> TQELGNANFENFIGATEGFSEIAYQFTSHILTLGYAVMLAGLLYFILTIKNVDKKFQMSNILSAVVMVSAFLLLYAQAQNWTSSFTFNEEVGRYFLDPSGDLFNNGYRYLNWLINVPMLLFQILFVVSLTTSKFSSVRNQFWFSGAMMIITGYIGQFYEVSNLTAFLVWGAISSAFFFHILWVMKKVINEGKEGISPAGQKILSNIWILFLISWTLYPGAYLMPYLTGVDGFLYSEDGVMARQLVYTIADVSSKVIYGVLLGNLAITLSKNKEL

Microbial rhodopsins (MRs) are transmembrane light-sensitive proteins, found in Archaea, Bacteria, Eukaryota, and also viruses. MRs are composed of seven transmembrane α-helices (A–G) with the cofactor retinal covalently bound to the lysine residue of helix G via the Schiff base (RSB). Despite this paradigm, the first light-driven Na+ pump KR2 was identified in Krokinobacter eikastus in 20132. KR2 contains a characteristic for all known Na+-pumping rhodopsins (NaRs) set of N112, D116, Q123 residues in the helix C (NDQ motif).

Moreover, it was recently reported that in the ground state under physiological conditions (PDB ID: 6REW4) KR2 has a large water-filled cavity near the RSB (Schiff base cavity). This conformation of the protein was called ‘expanded’, and only occurs in the pentameric form of KR2. On the contrary, in the monomeric form the large cavity is absent, and the protein is in another conformation, called ‘compact’. Thus, we suggest that neutralization of D116 is the key determinant of the formation of the ‘compact’ conformation, which explains their structural similarity.> ADKLFINALKKKFEESPEEKKTTFYTLGGWKQSERKTEFVNAGKEVAAKRGIPQYNPDIGTPLGQRVLMPYQVSTTDTYVEGDDLH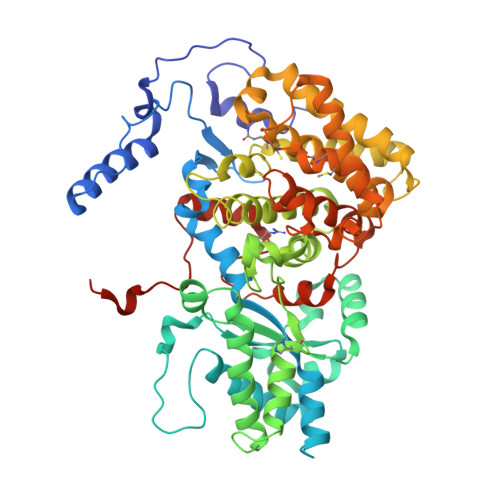FVNNAAMQQMWDDIRRTVIVGLNHAHAVIEKRLGKEVTPETITHYLETVNHAMPGAAVVQEHMVETHPALVADSYVKVFTGNDEIADEIDPAFVIDINKQFPEDQAETLKAEVGDGIWQVVRIPTIVSRTCDGATTSRWSAMQIGMSMISAYKQAAGEAATGDFAYAAKHAEVIHMGTYLPVRRARGENEPGGVPFGYLADICQSSRVNYEDPVRVSLDVVATGAMLYDQIWLGSYMSGGVGFTQYATAAYTDNILDDFTYFGKEYVEDKYGLCEAPNNMDTVLDVATEVTFYGLEQYEEYPALLEDQFGGSQRAAVVAAAAGCSTAFATGNAQTGLSGWYLSMYLHKEQHSRLGFYGYDLQDQCGASNVFSIRGDEGLPLELRGPNYPNYAMNVGHQGEYAGISQAPHAARGDAFVFNPLVKIAFADDNLVFDFTNVRGEFAKGALREFEPAGERALITPA> MAAVFGIQLVPKLNTSTTRRTFLPLRFDLLLDRLQSTNLHGVLYRALDFNPVDRSATVIQTYPPLNAWSPHHAFIENPLDYRDWTEFIHDRALAFVGVLTQRYPLTQNAQRYTNPLVLGAAFGDFLNARSIDIFLDRLFYDPTQDSPITAITKFPYQWTIDSNVTTDSVRTSAGCKYITLYGYDPSRPSTPATYGKHRPTYATVFYYSTLPARSRLLANLAAGPTVLEHFDSPTYGPHLLLPQTGDVLGYSSSLISQAALLMVESVMDALRDNANASASTAVTRLDQSYHPVTSFDPSTFNTLLQRATNLALLAVQGVQSESAIPAIPTMSDVRSFVARLMAEGDPQQWFPYRVDQILYWPESPFVPPIGPFYAPFRPVNFPFTTGSYTVVPDASRPLRLLPQYRNATITVQQADDAYEDTALSPLITTHGFCVTGGVFTSIYDISGDPTAYPPAQLVDAPNDYFDRERMARRDLFRRLRAPADRSAIKDRAVFDFLASLVNPTTANPVLDTSFSMAYLGASSAHANADEPVILADIRSGSIPGLPIPRRIVQFGYDVVHGSLLDLSRAVPTGTFGLVYADLDQVEDAGTDMPAANRAAIAMLGTALQMTTAGGVSVLKVNFPTRAFWTQVFNLYATHATTLHLVKPTIVNSSEVFLVFGGRQSNGALRSTTALQRALLSLYARNAAIDRAVTHIPFFGVPDDGTSDLGIDAVRLFDPMFSDAVANLPSNALASLVSRVVPSSIMFTRVPSNGPVSTTIYGKRTFLSNRRRARLRDVPMLITTTLVHQRRFTTPPTFTLFSSEAVPVTTLVAAGYNSFISEQTRNPNLAHLLDLGTGPECRILSLIPPTLQVTMSDSRPCAELMASFDPALTAYVQGDYSTAAFWNGIRCDSATAIFTIGAAAAAAGTDLIAFVQQLIPRIVAAGGTRMWLQLNTPLYEVSSLPDLIEIDLRDHVYRFNGGERVEPYADPVPLQQAIAALLPAAALSWHTLSPTCDWLPYIIGVGSPLNLSDINTAISYSRLTPILHIDTTTPPLRVNPVPTPLNQQCAIRITSLDPAAVLSVQHNGVEVIGGTPGNVISVAGAAALQYILANQEFLLQFTPTLPGIFDVFLTTLGQPPVPRGSFTITPPPTTVALNMPPPRQLDFTDVGNDARITCDPYYQLAVCIFKDGQYVRVNPEKASVVTNAPNRDLHFVLDLADNHVLLYLCDVTPSGLGDRIAFPIVDIYRIAFPRNTPVRASLPYTGGGAHLTSGGNPFMSLTTPPAVLPAGVALAALSTSVATQYPTYTLPAGVYEYVIE;> ANGPELIIEDTGLCTSFMLLDNIPSAHLTKELIGFTWFMQMYQMTPPLPEGAVNRIVCMTNWASLGDEGRGLEVRLPPPTDSSVHAYKTVLSRGYIDNAQFNPLALRSNVLLMLLQFTLSNLKINKSSTFTSDVTTITSGRMIRAFEGRPELLALAYPGRAVLPTQTKNAQFLSTAIADRIGRLDRANLIGGEVSAMVECMELCDALTLHIRETYIMLLRSMHQDPTQIVQIVNECANNLLNSTIPISLRPTILCPWFASSEDLRLQEVMHLVNISSNTAAALPLVEALSTLLRSVTPLVLDPTVLTNAITTISESTTQTISPISEILRLLQPMGNDYAAFWKCIASWAYNGLVTTVLSEDAFPDSSQSITHLPSMWKCLFLTLAGPMTSDPHSPVKVFMALANLLAQPEPIAIGVPGMHQTTPASQFSHPGVWPPGFLNPQLINPQQAPLLRAFAEHIRANWPQPSEFGYGSTLQGSANLFIPSNRMVYPWPNQPLPRLTVAPTYDSAMSNWISTTIAFFIRVVNSVNMTATVNDLTRRTMTGVMTAMRQVKTMTPFYIQHMCPTELSVLASVTVTPPFQVPFTRLVQNDVITNVLVARVDPAQRGDAAVDIRATHATFAAALPVDPAAIVVAMLCGQTETNLIPSHHYGKAFAPLFASNAMFTRNQRAVITREAFVCARSAVAQCQDAGFLVPRPLDALRQFDVTSAAAAEIMHAVNDAFKTAFDLDGALLDGLALYGDPRIADLSAAYLQYGGNVVREHVPPGPSHIHRALQQVESTFMAEMNLFNVARGNLYLVQTATNGNWSPMAPVAAPPFVRGGPNVRVVGRFGTIVPRPNGLEPQLIDDGNVPRDIAGDWVYPSDVLQVSVAVFRDYVWPMVKAGRTRVLVELGHYVYTLHYYDPQISLDEAPILEEWLSKINPAGIPPVPFCIPIPQVYPCITARRVHYAFTSENNNDSLFSTNAASIDTAFGENAAVSPLRWPGLVDPNYRVGTNDLPNRITLYNSLYRYNFTYPTLDGIMYVRSAT;> TNVVPAKDAPTTNSPPSTTSPNQAAADANQQQAGIVSSQSGPNAVGDSAPSSSVNNDGDIITRPTSDSIAAVANATKPAAVVSDPQSMKVTPIVNPSSYVCNVCNARFSTMSALSEHLRSDHRDDASTLLATPMINNAIRSFLTAWDDIRILSPDVSSKSLSAYLDSAVANGPELIIEDTGLCTSFMLLDNIPSAHLTKELIGFTWFMQMYQMTPPLPEGAVNRIVCMTNWASLGDEGRGLEVRLPPPTDSSVHAYKTVLSRGYIDNAQFNPLALRSNVLLMLLQFTLSNLKINKSSTFTSDVTTITSGRMIRAFEGRPELLALAYPGRAVLPTQTKNAQFLSTAIADRIGRLDRANLIGGEVSAMVECMELCDALTLHIRETYIMLLRSMHQDPTQIVQIVNECANNLLNSTIPISLRPTILCPWFASSEDLRLQQVMHLVNISSNTAAALPLVEALSTLLRSVTPLVLDPTVLTNAITTISESTTQTISPISEILRLLQPMGNDYAAFWKCIASWAYNGLVTTVLSEDAFPDSSQSITHLPSMWKCLFLTLAGPMTSDPHSPVKVFMALANLLAQPEPIAIGVPGMHQTTPASQFSHPGVWPPGFLNPQLINPQQAPLLRAFAEHIRANWPQPSEFGYGSTLQGSANLFIPSNRMVYPWPNQPLPRLTVAPTYDSAMSNWISTTIAFFIRVVNSVNMTATVNDLTRRTMTGVMTAMRQVKTMTPFYIQHMCPTELSVLASVTVTPPFQVPFTRLVQNDVITNVLVARVDPAQRGDAAVDIRATHATFAAALPVDPAAIVVAMLCGQTETNLIPSHHYGKAFAPLFASNAMFTRNQRAVITREAFVCARSAVAQCQDAGFLVPRPLDALRQFDVTSAAAAEIMHAVNDAFKTAFDLDGALLDGLALYGDPRIADLSAAYLQYGGNVVREHVPPGPSHIHRALQQVESTFMAEMNLFNVARGNLYLVQTATNGNWSPMAPVAAPPFVRGGP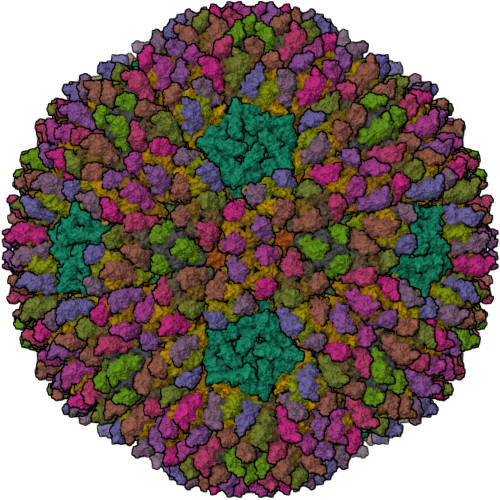NVRVVGRFGTIVPRPNGLEPQLIDDGNVPRDIAGDWVYPSDVLQVSVAVFRDYVWPMVKAGRTRVLVELGHYVYTLHYYDPQISLDEAPILEEWLSKINPAGIPPVPFCIPIPQVYPCITARRVHYAFTSENNNDSLFSTNAASIDTAFGENAAVSPLRWPGLVDPNYRVGTNDLPNRITLYNSLYRYNFTYPTLDGIMYVRSAT;>MAQRQFFGLTYNFYGQPAPLFDLNDLQELAGCYARPWTSRFSHLAISTGSLPVWSARYPSVASRNIVVNTLLGAHLNPFAGGQITSHQGITWRDPVLSSLAPVPAIQPPPVWAVAENVLLDSNNYPTYVLNLSSMWPINQDVHIMTMWALSDQGPIYHLEVPVDPMPAATTAALMAYTGVPIAHLAQTAYRFAGQLPQSPDSTMVSTIRWLSAIWFGSLTGRLNRSRTCNGFYFEFAKPALNPDQAVLKWNDGARAAPPAAAQSSYIRCISPHWQHQIVEVAGALMSQSVTAVTGLPALIDEATLPAWSQGVANLTGNGQGVVPCLDYNPVPMAAARHLQWRQDGLITAAQEAQLNNDYTAYALTIERHLTAMLVANPIAAGRMPIQPFNAADFGQAGQTAAAVALAQAMFV[2x];>MPLHMIPQVAHAMVRAAAAGRLTLYTRTRTETTNFDHAEYVTCGRYTICAFCLTTLAPHANVKTIQDSHACSRQPNEAIRSLVEVSDKAQTALVGSRTVDYHELDVKAGFVAPTADETIAPSKDIVELPFRTCDLDDSSATACVRNHCQAGHDGVIHLPILSGDFKLPNEHPTKPLDDTHPHDKVLTRCPKTGLLLVHDTHAHATAVVATAATRAILMHDLLTSANADDGHQARSACYGPAFNNLTFACHSTCASDMAHFDCGQIVGLDLHVEPSD[10x];>[10x]TYNITGDGNSFTPTSDMTSTAAPAIDLKPGVLNPTGKLWRPVGTSVATIDSLAIVSDRFGQYSFVNEGMRETFSKALFDINMWQPLFQATKTGCGPIVLSSFTTTTSGYVGATAGDALDNPVTNGVFISTVQIMNLQRTIAARMRDVALWQKHLDTAMTMLTPDISAGSASCNWKSLLAFAKDILPLDNLCLTYPNEFYNVAIHRYPALKPGNPDTKLPDAQAHPLGEVAGAFNAATSEVGSLVGSSSTLSQAISTMAGKDLDLIEADTPLPVSVFTPSLAPRSYRPAFIKPEDAKWIAEFNNSSLIRKTLTYSGATYTVQLGPGPTRVIDMNAMIDSVLTLDVSGTILPYDTNPDLSTSVPAFVLIQTSVPIQQVTTAANITAITVVSAAGASAINLAINVRGQPRFNMLHLQATFERETITGIPYIYGLGTFLIPSPTSSSNFSNPTLMDGLLTVTPVLLRETTYKGEVVDAIVPATVMANQTSEEVASALANDAIVLVSNHLNKLANVVGDAIPVASRTDDSATSAIVSRLAVQHKLSQVGQASPTPPDYPLLWRRAKRAASMFVSNPSLALQVGIPVLTQSGMLSALTSGVGTALRTGSLGKGVTDASEKLRARQSLTVAKQAFFDQIGSLWPGK>MDEALIKDYHSIREQIDQYTKDMVLVMQHPTNCVKYINPGRLMHVVTSDGTDFGWGVIINFYERRPERNNPNPGWSPQESYVVEVLLRLSSDSGSVDSKLKDNQCIPAGIAPVTQKNDPGRWEVVPCLLSCMHGLSQIKLHVPDKKSGGSMDDPETRRRVGKSLLEVQRRFEDGIPHMDPIENMHIRDVEFKKLLRKIEVLESRLVANPLHNS[2x];>GAMALSYSSPLRFFRNFRFHPEFTRLVAGGWRSLTYSSRIDPDKEMCPYELEGTQCPSGCSFQH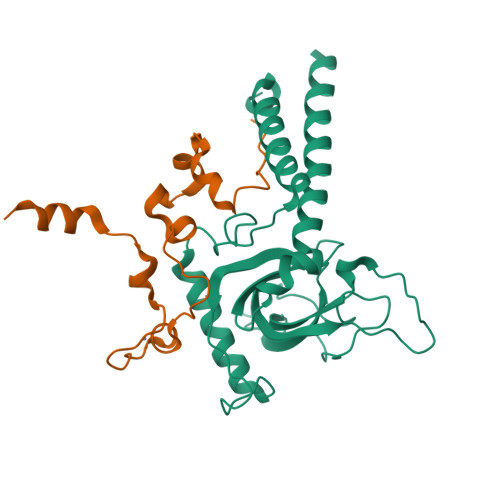FVDITPAADERILLELSGSHHHHHH[2x]> MSKAMALRRLMKEYKELTENGPDGITAGPSNEDDFFTWDCLIQGPDGTPFEGGLYP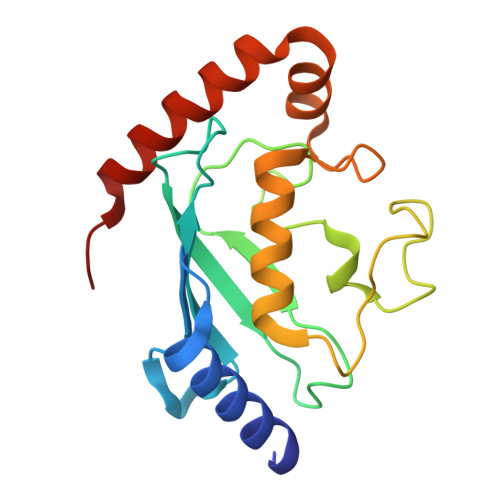ATLKFPSDYPLGPPTLKFECEFFHPNVYKDGTVCISILHAPGDDPNMYESSSERWSPVQSVEKILLSVMSMLAEPNDESGANIDACKMWREDREEYCRVVRRLARKTLGLLVPR>[3x]MSTVGTGKLTRAQRRAAARKNKRNTRVVQPVIVEPIASGQGKAIKA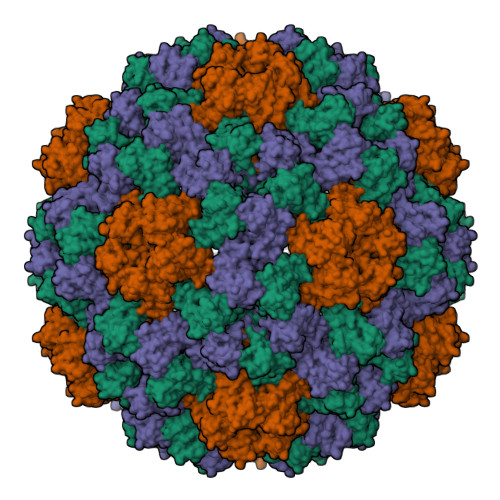WTGYSVSKWTASCAAAEAKVTSAITISLPNELSSERNKQLKVGRVLLWLGLLPSVSGTVKSCVTETQTTAAASFQVALAVADNSKDVVAAMYPEAFKGITLEQLTADLTIYLYSSAALTEGDVIVHLEVEHVRPTFDDSFTPVY>MELCHKTVKSRTAYSKHFPHKCQLPLGHSGKCLEFPFLVSLSKTHPRIAAKIVRDATMTTGAAWKSSQAGPNRMPRYVAILDDDILLEKFNLDMQSLPEITRLKIREKAADYDSCIDVARKLTWLAYQLHGAPIPDSFTKNYLEEFFGPMVAGSTNCEICKLPLTIDLFSENRVGKAAVETAHKTPRLHNAENVGFAHRFCNVAQGNKSLDEFYLWMEEVLTRVKML[4x]

DraIII is a type IIP restriction endonucleases (REases) that recognizes and creates a double strand break within the gapped palindromic sequence CAC↑NNN↓GTG of double-stranded DNA (↑ indicates nicking on the bottom strand; ↓ indicates nicking on the top strand). DraIII is a type IIP REase isolated from Deinococcus radiophilus ATCC 27603. However, wild type DraIII shows significant star activity. It indicated, as supported by mutagenesis, that DraIII possesses a ββα-metal HNH active site.

The structure of DraIII was determined in the presence of an 11-bp canonical DNA duplex containing a phosphorothioate at both of the scissile phosphodiester bonds. A complete protein structure was derived from a protein-phosphorothioate DNA duplex in the presence of magnesium chloride, although the DNA was not observed in the structure. DraIII exists as a homodimer and dimerization occurs in the C-terminus region where the ββα-metal HNH active site is located. Two zinc- and one magnesium-binding sites are found in each DraIII monomer. The DraIII monomer contains a ββα-metal fold (β1-β2-α12) in the C-terminal domain where the HNH active site is located. The N-terminal zinc binding site (consisting of C4, C22, H28 and C32) and the C-terminal zinc binding site (C157, C160, H198 and C201) of DraIII deviate from the CXXC/CXXC configuration. The DraIII structure is composed of two domains: the N-terminal domain (α1–9) and the C-terminal domain (α10–13, β1–2). More importantly, the domain interface opens up to the active site tunnel the substrate DNA would bind to (surface mode). Six potential hydrogen bonds are found between the two domains along the domain interface, which can be divided into three regions: the mouth, middle and hinge region. Among the known HNH REases, the structure presented here is the first for one that recognizes a gapped sequence.>MHHHHHHITSLYKKAGFMSNEYVALITARGGSKGLLRKNVLPLHGIPLIGWTIKAAQG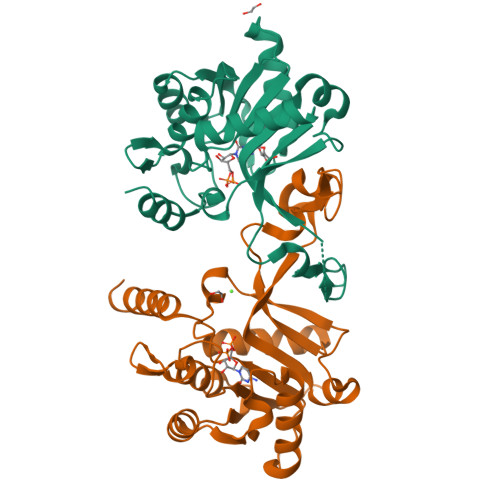CSYISKVFVSTDDYEIAKISEGLGALVINRPEELATDTASSIDVILHAISWLEQKEVQKYEGMILLQPTSPLRTSHHIKEAIELYEKTAAKFVISVFEPTHTPIKSYLENDDGTISGLYSNEAPYQRRQDLPRAYQPNGAIYAFSIDEFKLNNHFPRNKVFPYVMSEVESADIDTLEDLRKVEEQLKIKEINK[4x]> GDELYRQSLEIISRYLREQATGAKDTKPMGRSGATSRKALETLRRVGDGVQRNHETAFQGMLRKLDIKNEDDVKSLSRVMIHVFSDGVTN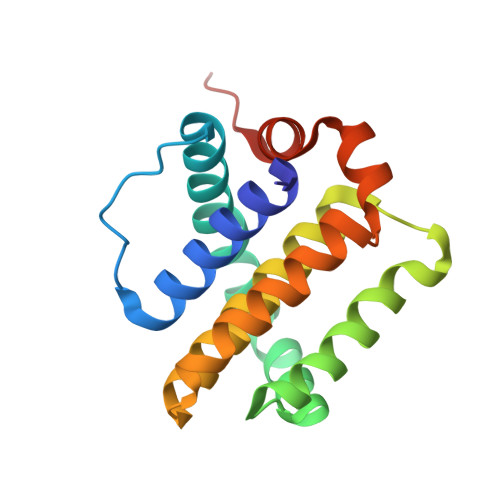WGRIVTLISFGAFVAKHLKTINQESCIEPLAESITDVLVRTKRDWLVKQRGWDGFVEFFHVEDLEGG> VNFEEVRELVPQKYPFLFIDKVIEL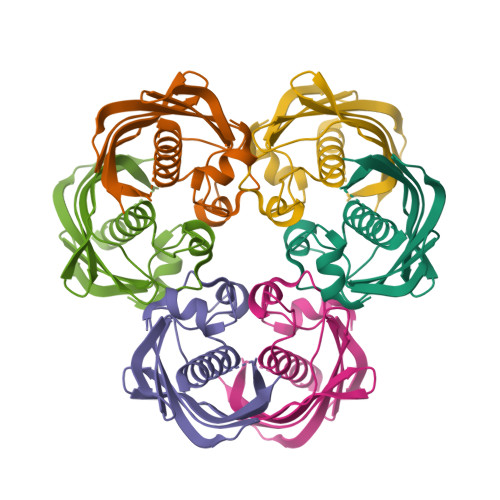QKEARIVCLKNISGNEPFFAGHFPDFAIMPGVLIVEALAQASGILFKKSFSTEQHKDDVFLLASANVRFSKPVFPGDQLILEIDIEKVISSAAIVKGVAKVGDKVVTKATLSFGVA> NEGKALMAIKGSFSNLVNMLLDWDDVHN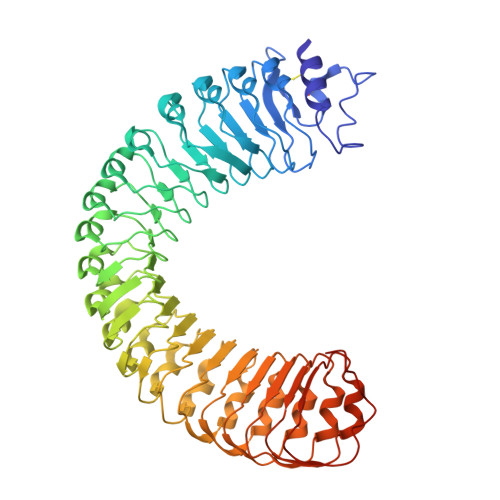SDLCSWRGVFCDNVSYSVVSLNLSSLNLGGEISPAIGDLRNLQSIDLQGNKLAGQIPDEIGNCASLVYLDLSENLLYGDIPFSISKLKQLETLNLKNNQLTGPVPATLTQIPNLKRLDLAGNHLTGEISRLLYWNEVLQYLGLRGNMLTGTLSSDMCQLTGLWYFDVRGNNLTGTIPESIGNCTSFQILDISYNQITGEIPYNIGFLQVATLSLQGNRLTGRIPEVIGLMQALAVLDLSDNELVGPIPPILGNLSFTGKLYLHGNMLTGPIPSELGNMSRLSYLQLNDNKLVGTIPPELGKLEQLFELNLANNRLVGPIPSNISSCAALNQFNVHGNLLSGSIPLAFRNLGSLTYLNLSSNNFKGKIPVELGHIINLDKLDLSGNNFSGSIPLTLGDLEHLLILNLSRNHLSGQLPAEFGNLRSIQMIDVSFNLLSGVIPTELGQLQNLNSLILNNNKLHGKIPDQLTNCFTLVNLNVSFNNLSGIVPPMANFSRFAPASFVGNPYLCGNW>[3x]MIKIKLTHPDCMPKIGSEDAAGMDLRAFFGTNPAADLRAIAPGKSLMIDTGVAVEIPRGWFGLVVPRSSLGKRHLMIA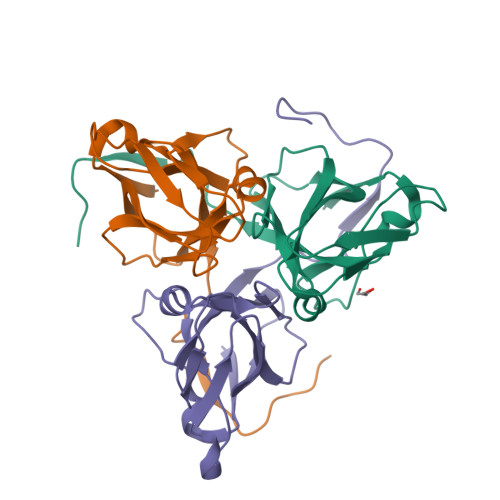NTAGVIDSDYRGTIKMNLYNYGSEMQTLENFERLCQLVVLPHYSTHNFKIVDELEETIRGEGGFGSSGSK>[7x]MSSKSDDFGSIVASGVTGSGDGNGNGNDWVEKAKDVLQTSVDAVTETAKKTKDVSDEMIPHVQQFLDSNPYLKDVIVPVSLTMTGTLFAWVVMPRILRRFHTYAMQSSAKLLPVGFSNEDVPYEKSFWGALEDPARYLVTFIAFAQIAAMVAPTTIAAQYFSPTVKGAVILSLVWFLYRWKTNVITRMLSAKSFGGLDREKVLTLDKVSSVGL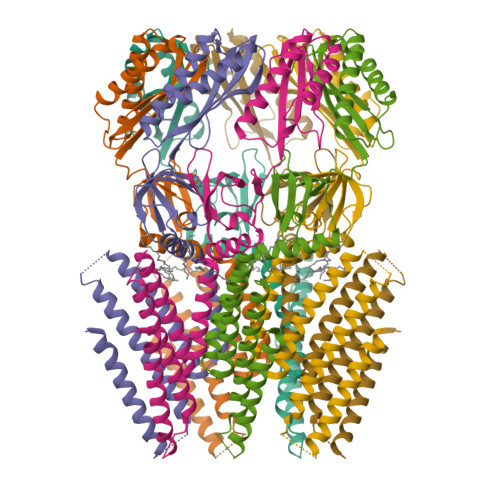FAIGLMASAEACGVAVQSILTVGGVGGVATAFAARDILGNVLSGLSMQFSRPFSMGDTIKAGSVEGQVIEMGLTTTSLLNAEKFPVLVPNSLFSSQVIVNKSRAQWRAIASKIPLQIDDLDMIPQISNEIKEMLRSNTKVFLGKEAPHCYLSRVEKSFAELTIGCNLIRMGKEELYNTQQEVLLEAVKIIKKHGVSLGTTWDNSTLSNSLEVLFQ>[9x]MLTNSEKSRFFLADLTGEVQSIPNTYGYISGLGLFRSAPQTQTTFLMDLTDWDISLLDAVDRTSRKAETSAPERVRQISFPMMYFKEVESITPDEIQ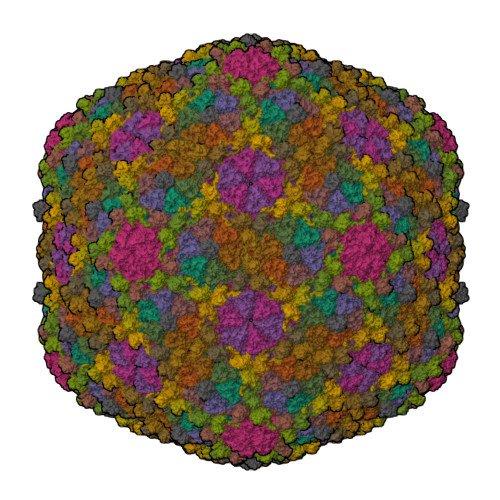GVRQPGTANELTTEAVVRAKKLMKIRTKFDITREFLFMQALKGKVIDANGVLYADLYKQFDVTKKTIYFDLDNPNSDIDAHIEDLRMHMEDEAKTGTVINGEEIHIVVDRTFFSKLIKHPKIRDAYLAQQTPLAWQQITGSLRTGGTDGVQAHMNRFYYGGVVFVQYNGKFKDKRGKTHTLVSIDGVSDTNVGVGHAFPNVAMLGEANNIFEVAYAPCPKMGYANTLGQELYVFEYEKDRDEGIDFEAHSYMLPYCTRPQLLVDVRSDAE;>MAYQGFTKLGEREPLNDIILWEEITPTGHSRKEYAPVASTEYRVGEVLKADGSKVAAGQEAQADSVCIVNFYADLQLSYHGQLKVVGIYRDAELKDLLKLESGVDAAAVKSALKAKGIDFVPTGL[9x];> MIKAKTYPDFKEFVKDFVANVKAGKRYDFRKYQEAVLPLTYSSPWPESDIPEVTDFNYTPDYTVPFSEELLYSVGAQMRTADFFMDLQYAIINGKDVDTVYCEWLARVKPFSMLNAKLKDSAQPPVITTQPTGGAVNEGSAINLSIVATNATSYQWKKGSSDISGATSATYTKAGAVPADAGSYTCVVTNDVGSTTSDAAVITINPLPVITTQPTSKAVNESSTLTLSVVATGATSYQWKKNGTNISGATSATYSKANAKTTDAGSYTCVVTNAVGSVTSNAATVTINPLPVITVQPQDQDLTVGQTLTISITATGATGYQWRKGNSNISGATSATYTKASVTTADDGNYDCVVTNAVGSVTSHQAKVQVTA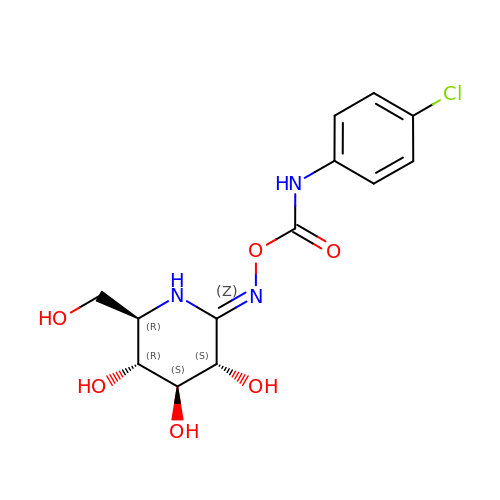[[(3S,4S,5R,6R)-3,4,5-trihydroxy-6-(hydroxymethyl)piperidin-2-ylidene]amino] N-(4-chlorophenyl)carbamate | C13 H16 Cl N3 O6 | TZXVKBJPSZOBNV-CHWFTXMASA-N>GQDMVSPPPPIADEPLTVNTGIYLIECYSLDDKAETFKVNAFLSLSWKDRRLAFDPVRSGVRVKTYEPEAIWIPEIRFVNVENARDADVVDISVSPDGTVQYLERFSARVLSPLDFRRYPFDSQTLHIYLIVRSVDTRNIVLAVDLEKVGKNDDVFLTGWDIESFTAVVKPANFALEDRLESKLDYQLRISRQYFSYIPNIILPMLFILFISWTAFWSTSYEANVTLVVSTLIAHIAFCILVETNLPKTPYMTYTGAIIFMIYLFYFVAVIEVTVQHYLKVESQPAR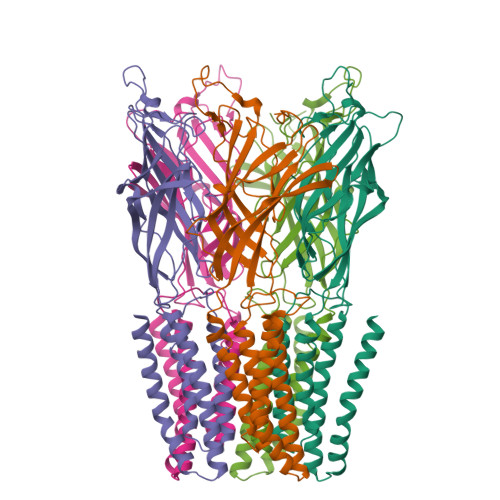AASITRASRIAFPVVFLLANIILAFLFFGF[5x]>MNIDVEFHI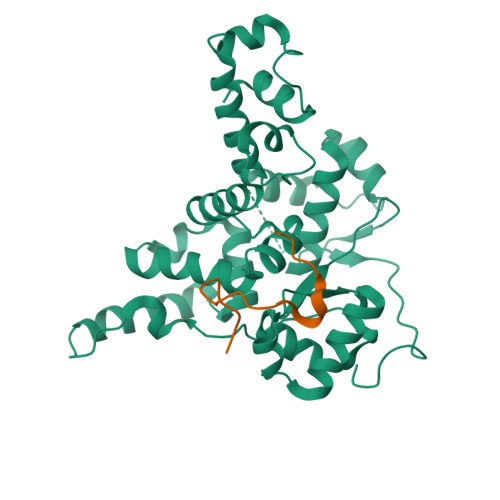RHNYPWNKLPANVRQSLGNSQREYEKQVVLYSIRNQLRYRNNLVKHVKKDERRYYEELLKYSRDHLMLYPYHLSDIMVKGLRITPFSYYTGIMEDIMNSEKSYDSLPNFTAADCLRLLGIGRNQYIDLMNQCRSSKKFFRRKTARDLLPIKPVEIAIEAWWVVQAGYITEDDIKICTLPEKCAVDKIIDSGPQLSGSLDYNVVHSLYNKGFIYLDVPISDDSCIAVPPLEGFVMNRVQGDYFETLLYKIFVSIDEHTNVAELANVLEIDLSLVKNAVSMYCRLGFAHKKGQVINLDQLHSSWK[2x];>[2x]RHVSSSDRVGKPYRGVKPVFS2,4-diamino-6-{[(1S)-1-(5-chloro-4-oxo-3-phenyl-3,4-dihydroquinazolin-2-yl)ethyl]amino}pyrimidine-5-carbonitrile 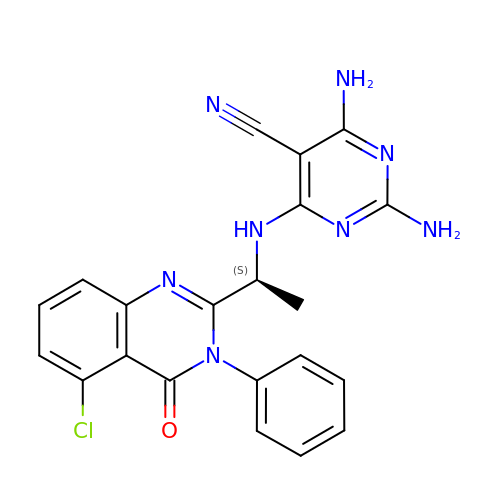| C21 H17 Cl N8 O | QQBVZBSMGUVONA-NSHDSACASA-N[(2~{R},3~{S},4~{R},5~{R})-5-(4-azanylpyrrolo[2,1-f][1,2,4]triazin-7-yl)-5-cyano-3,4-bis(oxidanyl)oxolan-2-yl]methyl dihydrogen phosphate | C12 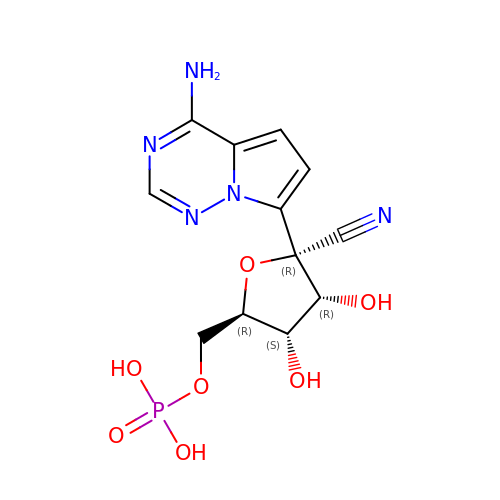H14 N5 O7 P | ZBHOHJWLOOFLMW-LTGWCKQJSA-N>MKLIILDRDGVVNQDSDAFVKSPDEWIALPGSLQAIARLTQADWTVVLATNQSGLARGLFDTATLNAIHDKMHRALAQMGGVVDAIFMCPHGPDDGCACRKPLPGMYRDIA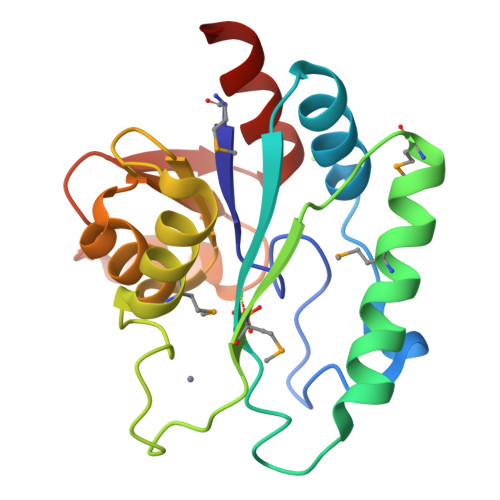RRYDVDLAGVPAVGDSLRDLQAAAQAGCAPWLVQTGNGRKTLAQGGLPEGTRVCEDLAAVAEQLLQEA[4x]(3aS)-3a-hydroxy-7-methyl-1-phenyl-1,2,3,3a-tetrahydro-4H-pyrrolo[2,3-b]quinolin-4-one | C18 H16 N2 O2 | 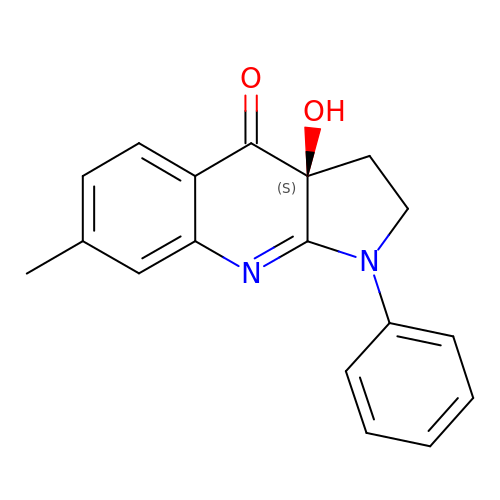KAJFGRLMKVNMLH-GOSISDBHSA-N>[21x]MITNNLVPTVIEKTAGGERAFDIYSRLLKERIVFLNGEVNDHSANLVIAQLLFLESEDPDKDIYFYINSPGGMVTAGMGVYDTMQFIKPDVSTICIG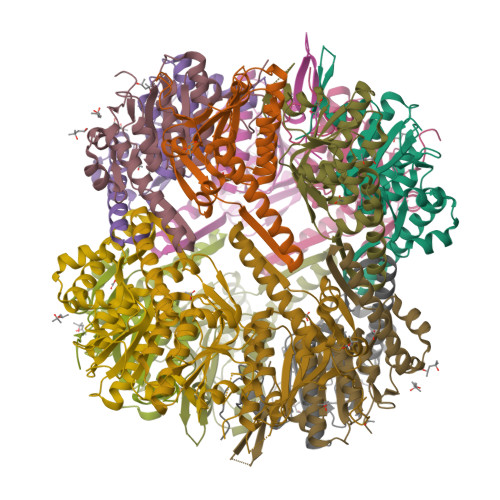LAASMGSLLLAGGAKGKRYSLPSSQIMIHQPLGGFRGQASDIEIHAKNILRIKDRLNKVLAHHTGQDLETIVKDTDRDNFMMADEAKAYGLIDHVIESREAIIK> ELTPDQQTLLHFIMDSYNKQRMPQEITNKILKEAFSAEENFLILTEMATNHVQVLVEFTKKLPGFQTLDHEDQIALLKGSAVEAMFLRSAEIFNKKLPSGHSDLLEERIRNSGISDEYITPMFSFYKSIGELKMTQEEYALLTAIVILSPDRQYIKDREAVEKLQEPLLDVLQKLCKIHQPENPQHFAKLLGRLTELRTFNHHHAEMLMSWRVDH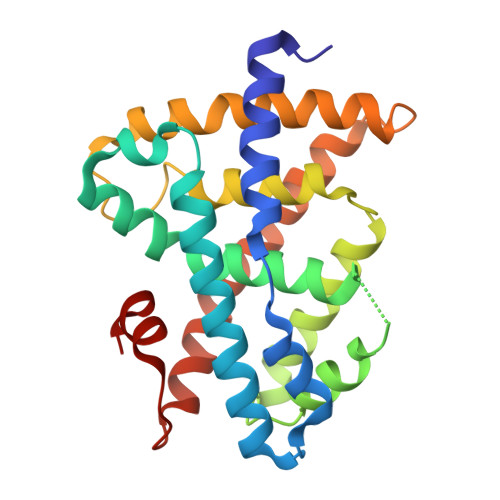KFTPLLQEIWDV>MAIAQLATEYVFSDFLLKEPTEPKFKGLRLELAVDKMVTCIAVGLPLLLISLAFAQEISIGTQISCFSPSSFSWRQAAFVDSYCWAAVQQKNSLQSESGNLPLWLHKFFPYILLLFAILLYLPPLFWRFAAAPHICSDLKFIMEELDKVYNRAIKAAKSARDLDMRDGACSVPGVTENLGQSLWEVSESHFKYPIVEQYLKTKKNSNNLIIKYISCRLLTLIIILLACIYLGYYFSLSSLSDEFVCSIKSGILRNDSTVPDQFQCKLIAVGIFQLLSVINLVVYVLLAPVVVYTLFVPFRQKTDVLKVYEILPTFDVLHFKSEGYNDLSLYNLFLEENISEVKS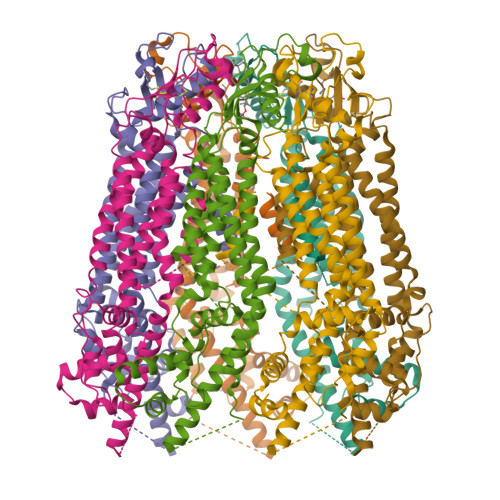YKCLKVLENIKSSGQGIDPMLLLTNLG[7x]>RILPDSVDWREKGCVTEVKYQGSCGACWAFSAVGALEAQLKLKTGKLVSLSAQNLVDCSTEKYGNKGCNGGFMTTAFQYIIDNKGIDSDASYPYKAMDQKCQYDSKYRAATCSKYTELPYGREDVLKEAVANKGPVSVGVDARH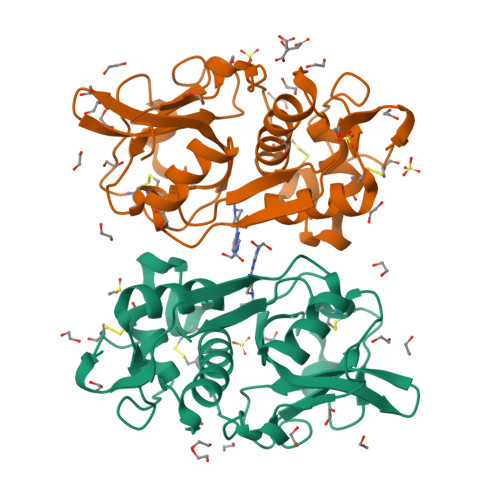PSFFLYRSGVYYEPSCTQNVNHGVLVVGYGDLNGKEYWLVKNSWGHNFGEEGYIRMARNKGNHCGIASFPSYPEIHHHHHH[2x]> ENYRRVVRGNQNQRPEFPPPRYNFTIVTTYNETS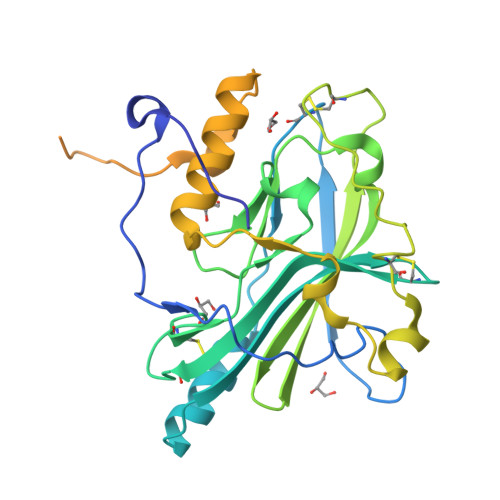LPSPFINDQVKIVDVRTVAATRPCEMIALIAKTNVDSIIKELDAAHKTYSARLTWFKITPTCATPIHDVVYMKCNPKLLFGMCDERSNILWLNSLITTAAETDDELGLVLASPAHSYSGLYRRVIQIDGRRIYTDFSVTIPSSHCPLSFEQNFGNPDRCKTPEQYSRGEVYTSRFLSEFNYRQGVHLAWVKHWFVQDGGNLPVQFYEAQAFARPVPPDNHPGFDSVESEITQNKTNPKQEQASPKPNPPFKWPSIKQLAPRIDEVDNAKEITTKKPPASNSNSTFENLYFQGHHHHHH> ANPHKDVLKGPFTTGSEVTTQCLTCHEEQATDMMKTSHWTWELEQKLPDRTVVRGKKNSINNFCVAISSNEPRCTSCHAGYGWKDNTFDFKDKTKVDCLICHDTTGTYVKDPAGAGEPMAKLDLAKIAQNVGAPVRDNCGSCHFYGGGGDAVKHGDLDSSMAYPDKATDVHMDSDGNNFQCQNCHTTEKHQISGNAMGVSPGGIDHIGCENCHDSAPHSNKKLNTHTATVACQTCHIP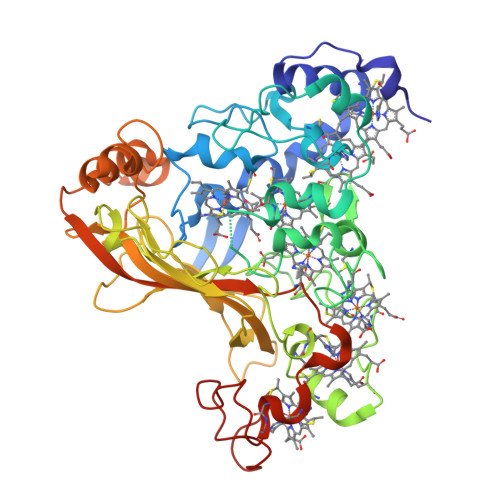FFAKNEPTKMQWDWSTAGDDKPETVDQYGKHTYQKKKGNFVWEKMVKPQYAWYNGTANAYMAGDKMDSNVVTKLTYPMGDINDAKAKIYPFKVHTGKQIYDKKLNIFITPKTYGKGGYWSEFDWNLAAKLGMEANPTMLEKGIKYSGEYDFAATEMWWRINHMVSPKEQALNCNDCHNKGTRLDWQALGYQGDPMKNKQGPKHKQ> MTLTERLREKISRAFYNHGLLCASYPIPIILFTGFCILACCYPLLKLPLPGTGPVEFTTPVKDYSPPPVDSDRKQGEPTEQPEWYVGAPVAYVQQIFVKSSVFPWHKNLLAVDVFRSPLSRAFQLVEEIRNHVLRDSSGIRSLEELCLQVTDLLPGLRKLRNLLPEHGCLLLSPGNFWQNDWERFHADPDIIGTIHQHEPKTLQTSATLKDLLFGVPGKYSGVSLYTRKRMVSYTITLVFQHYHAKFLGSLRARLMLLHPSPNCSLRAESLVHVHFKEEIGVAELIPLVTTYIILFAYIYFS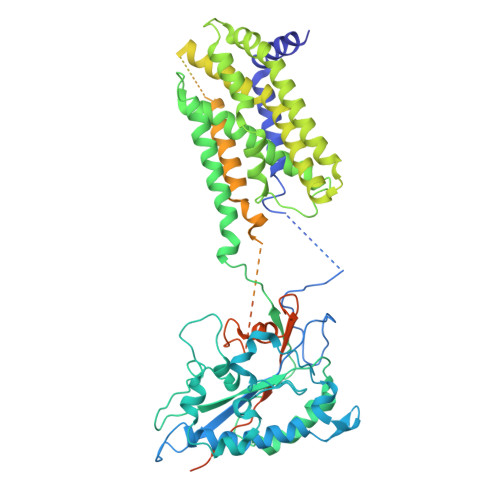TRKIDMVKSKWGLALAAVVTVLSSLLMSVGLCTLFGLTPTLNGGEIFPYLVVVIGLENVLVLTKSVVSTPVDLEVKLRIAQGLSSESWSIMKNMATELGIILIGYFTLVPAIQEFCLFAVVGLVSDFFLQMLFFTTVLSIDIRRMELADLNKRLPPEACLPSAKPVGQPTRYERQLAVRPSTPHTITLQPSSFRNLRLPKRLRVVYFLARTRLAQRLIMAGTVVWIGILVYTDPAGLRNYLAAQVTEQSPLGEGALAPMPVPSGMLPPSHPDPAFSIFPPDAPKLPENQTSPGESPERGGPAEVVHDSPVPEVTWGPEDEELWRKLSFRHWPTLFSYYNITLAKRYISLLPVIPVTLRLNPREALEGRHPQDGRSAWPPPGPIPAGHWEAGPKGPGGVQAHGDVTLYKVAALGLATGIVLVLLLLCLYRVLCP>[2x]MDRRALRIGVNGLPPSLEPINGISNTGPRIINQIFDALIRRDYFADGAKGNNIKLVPALAESFERIDDKSIRFKLRQGVKFHNGA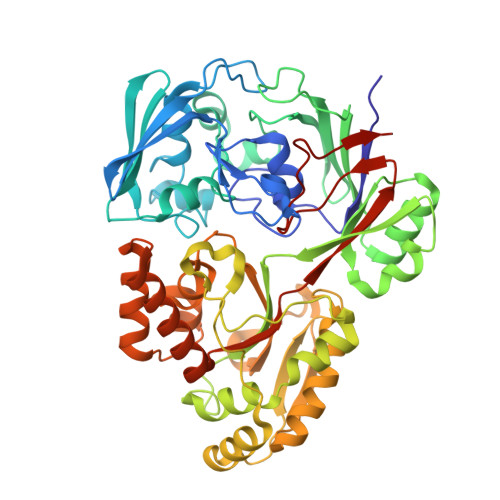EMTAEDVAFTFSSERLWGDEAIKTVPNGRNFSPNWDEPVVEDKYTVVLRTKTPSYLIEKYLGSWLGPIVPKEYYKSLGAVAFGNKPIGTGPYKFRELVANDHVTLEANDGYWGDKPTASTITYQVVAEPATRVAGLISGEYDIITTLTPDDMALVDGYSDLETRGTLIENLHMFTFNMNQPIFQNKTLRRALALAVNRPLIVEALWKNKASIPNGFNFPHYGATYDPKRKPMEFNLKEAKRLVKESGYDGTPITYHTMGNYYANAVPALMMMIEMWKAAGITVVPKIFAPGTTPKDSDILIRNWSNGQWLTDGLTTMVSEFGPGRGVQKRWGWKAPAEFNNLCDQVAQLKDGEERSAAFNRLRDIFEDEAPAVLMYQPYDVYAARKDVQWSPVSFETMEFRGNLNFKHHHHHH>[2x]GSDACVHHIKRRDIVLKWELGEGAFGKVFLAECHNLLPEQDKMLVAVKALKEASESARQDFQREAELLTMLQHQHIVRFFGVCTEGRPLLMVFEYMRHGDLNRFLRSHGPDAKLLAGGEDVAPGPLGLGQLLAVASQVAAGMVYLAGLHFVHRDLATRNCLVGQGLVVKIGDFGMSRDIYSTDYYRVGG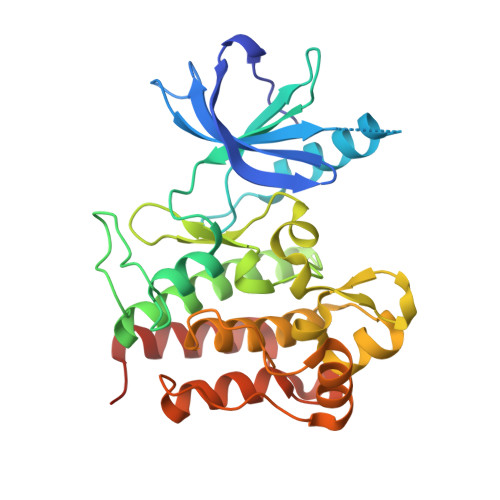RTMLPIRWMPPESILYRKFTTESDVWSFGVVLWEIFTYGKQPWYQLSNTEAIDCITQGRELERPRACPPEVYAIMRGCWQREPQQRHSIKDVHARLQALAQAPPVYLDVLG> XXXXXXXXXXXXXXXXXXXXXXXXXXXXXXXXXXXXXXXXXXXXXXXXXXXXXXXXXXXXXXXXXXXXXALETVGEKKAFSSVMQLVMTSLQSILENVDTPELLCKCVKCILLVARCYPHIFSTNFRDTVDILVGWHIDHTQKPSLTQQVSGWLQSLEPFWVADLAFSTTLLGQFLEDMEAYAEDLSHVASGESVDEDVPPPSVSLPKLAALLRVFSTVVRSIGERFSPIRGPPITEAYVTDVLYRVMRCVTAANQVFFSEAVLTAANECVGVLLGSLDPSMTIHCDMVITYGLDQLENCQTCGTDYIISVLNLLTLIVEQINTKLPSSFVEKLFIPSSKLLFLRYHKEKEVVAVAHAVYQAVLSLKNIPVLETAYKLILGEMTCALNNLLHSLQLPEACSEIKHEAFKNHVFNVDNAKFVVIFDLSALTTIGNAKNSLIGMWALSPTVFALLSKNLMIVHSDLAVHFPAIQYAVLYTLYSHCTRHDHFISSSLSSSSPSLFDGAVISTVTTATKKHFSIILNLLGILLKKDNLNQDTRKLLMTWALEAAVLMRKSETYAPLFSLPSFHKFCKGLLANTLVEDVNICLQACSSLHALSSSLPDDLLQRCVDVCRVQLVHSGTRIRQAFGKLLKSIPLDVVLSNNKHTEIQEISLALRSHMSKAPSNTFHPQDFSDVISFILYGNSHRTGKDNWLERLFYSCQRLDKRDQSTIPRNLLKTDAVLWQWAIWEAAQFTVLSKLRTPLGRAQDTFQTIEGIIRSLAAHTLNPDQDVSQWTTADNDEGHGNNQLRLVLLLQYLENLEKLMYNAYEGCANALTSPPKVIRTFFYTNRQTCQDWLTRIRLSIMRVGLLAGQPAVTVRHGFDLLTEMKTTSLSQGNELEVTIMMVVEALCELHCPEAIQGIAVWSSSIVGKNLLWINSVAQQAEGRFEKASVEYQEHLCAMTGVDCCISSFDKSVLTLANAGRNSASPKHSLNGESRKTVLSKPTDSSPEVINYLGNKACECYISIADWAAVQEWQNSIHDLKKSTSSTSLNLKADFNYIKSLSSFESGKFVECTEQLELLPGENINLLAGGSKEKIDMKKLLPNMLSPDPRELQKSIEVQLLRSSVCLATALNPIEQDQKWQSITENVVKYLKQTSRIAIGPLRLSTLTVSQSLPVLSTLQLYCSSALENTVSNRLSTEDCLIPLFSEALRSCKQHDVRPWMQALRYTMYQNQLLEKIKEQTVPIRSHLMELGLTAAKFARKRGNVSLATRLLAQCSEVQLGKTTTAQDLVQHFKKLSTQGQVDEKWGPELDIEKTKLLYTAGQSTHAMEMLSSCAISFCKSVKAEYAVAKSILTLAKWIQAEWKEISGQLKQVYRAQHQQNFTGLSTLSKNILTLIELPSVNTMEEEYPRIESESTVHIGVGEPDFILGQLYHLSSVQAPEVAKSWAALASWAYRWGRKVVDNASXXXXXXXXXXXXXXXXXXXXXXXXXXXXXXXXXXXXXXXXXXEGVIKVWRKVVDRIFSLYKLSCSAYFTFLKLNAGQIPLDEDDPRLHLSHRVEQSTDDMIVMATLRLLRLLVKHAGELRQYLEHGLETTPTAPWRGIIPQLFSRLNHPEVYVRQSICNLLCRVAQDSPHLILYPAIVGTISLSSESQASGNKFSTAIPTLLGNIQGEELLVSECEGGSPPASQDSNKDEPKSGLNEDQAMMQDCYSKIVDKLSSANPTMVLQVQMLVAELRRVTVLWDELWLGVLLQQHMYVLRR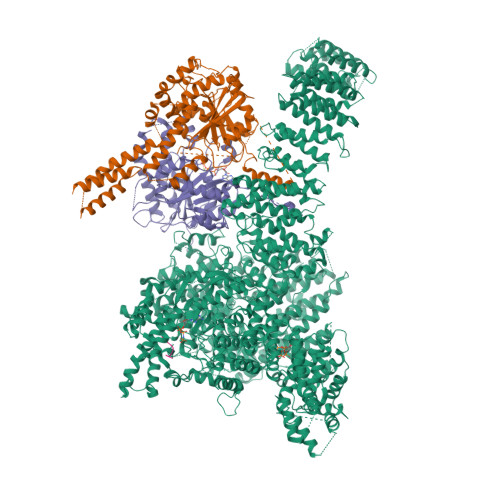IQQLEDEVKRVQNNNTLRKEEKIAIMREKHTALMKPIVFALEHVRSITAAPAETPHEKWFQDNYGDAIENALEKLKXXXXXXXXXXXXXXXXYILRLEEISPWLAAMTNTEIALPGEVSARDTVTIHSVGGTITILPTKTKPKKLLFLGSDGKSYPYLFKGLEDLHLDERIMQFLSIVNTMFATINRQETPRFHARHYSVTPLGTRSGLIQWVDGATPLFGLYKRWQQREAALQAQKAQDSYQTPQNPGIVPRPSELYYSKIGPALKTVGLSLDVSRRDWPLHVMKAVLEELMEATPPNLLAKELWSSCTTPDEWWRVTQSYARSTAVMSMVGYIIGLGDRHLDNVLIDMTTGEVVHIDYNVCFEKGKSLRVPEKVPFRMTQNIETALGVTGVEGVFRLSCEQVLHIMRRGRETLLTLLEAFVYDPLVDWTAGGEAGFAGAVYGGGGQQAESKQSKREMEREITRSLFSSRVAEIKVNWFKNRDEMLVVLPKLDGSLDEYLSLQEQLTDVEKLQGKLLEEIEFLEGAEGVDHPSHTLQHRYSEHTQLQTQQRAVQEAIQVKLNEFEQWITHYQAAFNNLEATQLASLLQEISTQMDLGPPSYVPATAFLQNAGQAHLISQCEQLEGEVGALLQQRRSVLRGCLEQLHHYATVALQYPKAIFQKHRIEQWKTWMEELICNTTVERCQELYRKYEMQYAPQPPPTVCQFITATEMTLQRYAADINSRLIRQVERLKQEAVTVPVCEDQLKEIERCIKVFLHENGEEGSLSLASVIISALCTLTRRNLMMEGAASSAGEQLVDLTSRDGAWFLEELCSMSGNVTCLVQLLKQCHLVPQDLDIPNPMEASETVHLANGVYTSLQELNSNFRQIIFPEALRCLMKGEYTLESMLHELDGLIEQTTDGVPLQTLVESLQAYLRNAAMGLEEETHAHYIDVARLLHAQYGELIQPRNGSVDETPKMSAGQMLLVAFDGMFAQVETAFSLLVEKLNKMEIPIAWRKIDIIREARSTQVNFFDDDNHRQVLEEIFFLKRLQTIKEFFRLCGTFSKTLSGSSSLEDQNTVNGPVQIVNVKTLFRNSCFSEDQMAKPIKAFTADFVRQLLIGLPNQALGLTLCSFISALGVDIIAQVEAKDFGAESKVSVDDLCKKAVEHNIQIGKFSQLVMNRATVLASSYDTAWKKHDLVRRLETSISSCKTSLQRVQLHIAMFQWQHEDLLINRPQAMSVTPPPRSAILTSMKKKLHTLSQIETSIATVQEKLAALESSIEQRLKWAGGANPALAPVLQDFEATIAERRNLVLKESQRASQVTFLCSNIIHFESLRTRTAEALNLDAALFELIKRCQQMCSFASQFNSSVSELELRLLQRVDTGLEHPIGSSEWLLSAHKQLTQDMSTQRAIQTEKEQQIETVCETIQNLVDNIKTVLTGHNRQLGDVKHLLKAMAKDEEAALADGEDVPYENSVRQFLGEYKSWQDNIQTVLFTLVQAMGQVRSQEHVEMLQEITPTLKELKTQSQSIYNNLVSFASPLVTDATNECSSPTSSATYQPSFAAAVRSNTGQKTQPDVMSQNARKLIQKNLATSADTPPSTVPGTGKSVACSPKKAVRDPKTGKAVQERNSYAVSVWKRVKAKLEGRDVDPNRRMSVAEQVDYVIKEATNLDNLAQLYEGWTAWV;> MAGPVSLRDLLMGASAWMGSESPGGSPTEGGGSAAGGPEPPWREDEICVVGIFGKTALRLNSEKFSLVNTVCDRQVFPLFRHQDPGDPGPGIRTEAGAVGEAGGAEDPGAAAGGSVRGSGAVAEGNRTEAGSQDYSLLQAYYSQESKVLYLLLTSICDNSQLLRACRALQSGEAGGGLSLPHAEAHEFWKHQEKLQCLSLLYLFSVCHILLLVHPTCSFDITYDRVFRALDGLRQKVLPLLKTAIKDCPVGKDWKLNCRPCPPRLLFLFQLNGALKVEPPRNQDPAHPDKPKKHSPKRRLQHALEDQIYRIFRKSRVLTNQSINCLFTVPANQAFVYIVPGSQEEDPVGMLLDQLRSHCTVKDPESLLVPAPLSGPRRYQVMRQHSRQQLSFHIDSSSSSSSGQLVDFTLREFLWQHVELVLSKKGFDDSVGRNPQPSHFELPTYQKWISAASKLYEVAIDGKEEDLGSPTGELTSKILSSIKVLEGFLDIDTKFSENRCQKALPMAHSAYQSNLPHNYTMTVHKNQLAQALRVYSQHARGPAFHKYAMQLHEDCYKFWSNGHQLCEERSLTDQHCVHKFHSLPKSGEKPEADRNPPVLYHNSRARSTGACNCGRKQAPRDDPFDIKAANYDFYQLLEEKCCGKLDHINFPVFEPSTPDPAPAKNESSPAPPDSDADKLKEKEPQTQGESTSLSLALSLGQSTDSLGTYPADPQAGGDNPEVHGQVEVKTEKRPNFVDRQASTVEYLPGMLHSNCPKGLLPKFSSWSLVKLGPAKSYNFHTGLDQQGFIPGTNYLMPWDIVIRTRAEDEGDLDTNSWPAPNKAIPGKRSAVVMGRGRRRDDIARAFVGFEYEDSRGRRFMCSGPDKVMKVMGSGPKESALKALNSDMPLYILSSSQGRGLKPHYAQLMRLFVVVPDAPLQIILMPQVQPGPPPCPVFYPEKQEITLPPDGLWVLRFPYAYVTERGPCFPPKENVQLMSYKVLRGVLKAVTQ;> MSESGHSQPGLYGIERRRRWKEPGSGGPQNLSGPGGRERDYIAPWERERRDASEETSTSVMQKTPIILSKPPAERSKQPPPPTAPAAPPAPAPLEKPIVLMKPREEGKGPVAVTGASTPEGTAPPPPAAPAPPKGEKEGQRPTQPVYQIQNRGMGTAAPAAMDPVVGQAKLLPPERMKHSIKLVDDQMNWCDSAIEYLLDQTDVLVVGVLGLQGTGKSMVMSLLSANTPEEDQRTYVFRAQSAEMKERGGNQTSGIDFFITQERIVFLDTQPILSPSILDHLINNDRKLPPEYNLPHTYVEMQSLQIAAFLFTVCHVVIVVQDWFTDLSLYRFLQTAEMVKPSTPSPSHESSSSSGSDEGTEYYPHLVFLQNKARREDFCPRKLRQMHLMIDQLMAHSHLRYKGTLSMLQCNVFPGLPPDFLDSEVNLFLVPFMDSEAESENPPRAGPGSSPLFSLLPGYRGHPSFQSLVSKLRSQVMSMARPQLSHTILTEKNWFHYAARIWDGVRKSSALAEYSRLLA;> QPELSQDSYLG>[4x]MASMSLKHFIQDALSSWMKQKGPESDIVLSSRIRLARNFEHIRFPTRYSNEEASSIIQQFEDQFSEQEIPGIGKFVLIRMNDAQPLEKRVLVEKHLISPNLTESPFGGCLLSENEEVSVMLNEEDHIRIQCLFPGFQLLEAMKAANQVDDWIEEKVDYAFNEQRGYLTSCPTNVGTGLRASVMMHLPALVLTRQINRIIPAINQLGLVVRGIYGEGSEAVGNIFQISNQITLGKSEQDIVEDLNSVAAQLIEQERSAREAIYQTSKIELEDRVYRSYGVLSNCRMIESKETAKCLSDVRLGIDLGIIKGLSSNILNELMILTQPGFLQQYSGGALRPNERDIRRAALIRERLHLEMNGKRQEDESILEHHHHHH

In Gram-positive bacteria, the McsB protein arginine kinase is central to protein quality control, labeling aberrant molecules for degradation by the ClpCP protease. McsB is a prominent member of the specialized bacterial kinases and has the unique activity of phosphorylating arginine residues. On a molecular level, the McsB kinase is composed of a specialized phospho-transferase scaffold for arginine phosphorylation and a dimerization domain aligning two subunits (Suskiewicz et al., 2019). Aside from this regulatory role, the phosphoarginine (pArg) mark introduced by McsB has a broader function in the cell, serving as a degradation tag that directs client proteins to the ClpC:ClpP protease (Stannek et al., 2014; Trentini et al., 2016).

We obtained crystals diffracting to 2.5 Å resolution, revealing the atomic structure of the McsBBS octamer. The octameric particle represents a tetramer of dimers, with each dimer resembling the reported McsBGS structure in its subunit contacts, domain arrangement and active site organization. The four McsBBS dimers form a molecular cage having the length of one dimer, 110 Å, and a diameter of 80 Å. The phosphorylation chamber has well-defined entrance gates with openings of approximately 25 Å. Potential substrates have to pass the entrance gates in order to reach the active sites, which are buried within the inner chamber. Octamer formation proceeds along the extended edge of the brick-shaped McsB dimer, where two clusters of polar residues enclose a small hydrophobic core. Strikingly, the electron density revealed that Arg194 is phosphorylated at a terminal amine of its guanidinium group. The pArg194 phospho-guanidinium group is accommodated in a complementarily charged pocket of a neighboring dimer. In the McsBBS octamer, Arg337*, Arg341*, and Ser285* of the molecular neighbor closely interact with the pArg194 phosphoryl group, whereas Asp338* tightly binds to the positively charged nitrogen of the pArg guanidinium function. It assembles into a self-compartmentalized kinase stabilized by the auto-phosphorylated residue pArg194.> GPLGSEIDYTAYPWFAGNMERQQTDNLLK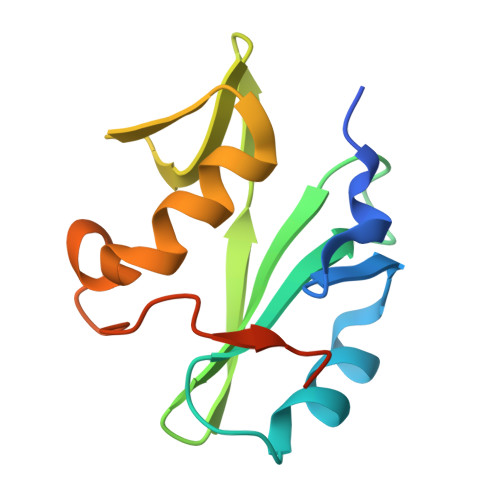SHASGTYLIRERPAEAERFAISIKFNDEVKHIKVVEKDNWIHITEAKKFDSLLELVEYYQCHSLKESFKQLDTTLKYPYKSRERSAGIL>[3x]MVCKVCGQKAQVEMRSRGLALCREHYLDWFVKETERAIRRHRMLLPGERVLVAVSGGKDSLALWDVLSRLGYQAVGLHIELGIGEYSKRSLEVTQAFARERGLELLVVDLKEAYGFGVPELARLSGRVACSACGLSKRYIINQVAVEEGFRVVATGHNLDDEAAVLFGNLLNPQEETLSRQGPVLPEKPGLAARVKPFYRFSEREVLSYTLLRGIRYLHEECPN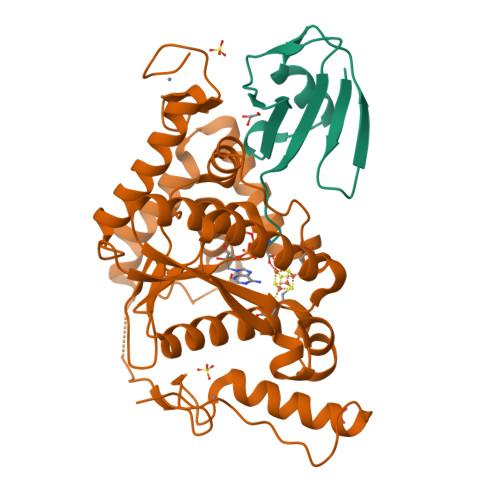AKGAKSLLYKEALNLVERSMPGAKLRFLDGFLEKIRPRLDVGEEVALRECERCGYPTTGAVCAFCRMWDAVYRRAKKRKLLPEEVSFRPRVKPLRAG;>MGSSHHHHHHRVVLRLPERKEVEVKGNRPLREVLEELGLNPETVVAVRGEELLTLEDEVREEDTLEVLSAISGG[3x]>[2x]SVVELGKMIIQETGKSPFPSYTSYGCFCGG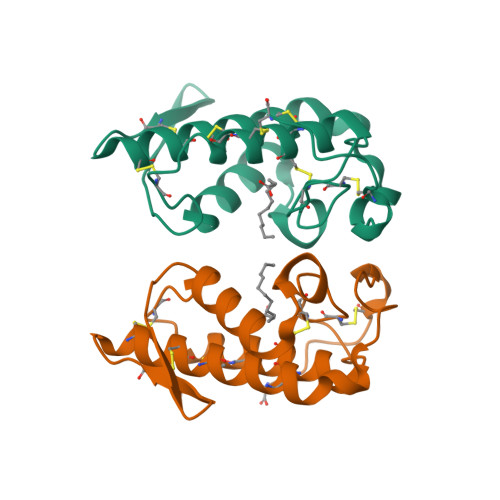GERGPPLDATDRCCLAHSCCYDTLPDCSPKTDRYKYKRENGEIICENSTSCKKRICECDKAVAVCLRKNLNTYNKKYTYYPNFWCKGDIEKC>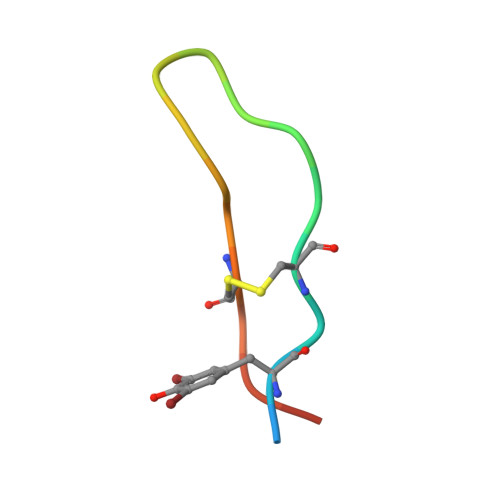 GGTYSCHFGPLTWVCKPQGG>[8x]SNAMSRKPFIAGNWKMNKNP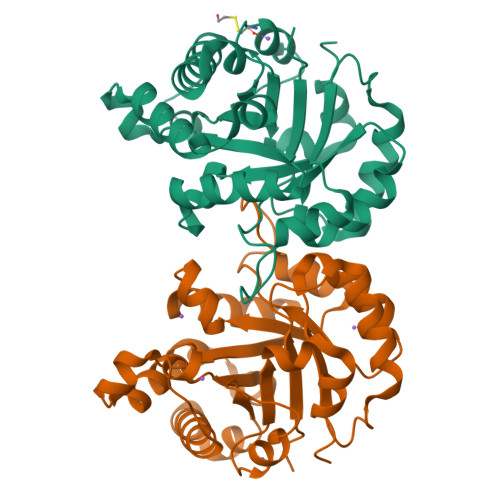EEAKAFVEAVASKLPSSDLVEAGIAAPALDLTTVLAVAKGSNLKVAAQNCYFENAGAFTGETSPQVLKEIGTDYVVIGHSERRDYFHETDEDINKKAKAIFANGMLPIICCGESLETYEAGKAAEFVGAQVSAALAGLTAEQVAASVIAYEPIWAIGTGKSASQDDAQKMCKVVRDVVAADFGQEVADKVRVQYGGSVKPENVASYMACPDVDGALVGGASLEAESFLALLDFVK> HMGAPATVTEQGEDITSKKDRGVLKIVKRVGNGEETPMIGDKVYVHYKGKLSNGKKFDSSHDRNEPFVFSLGKGQV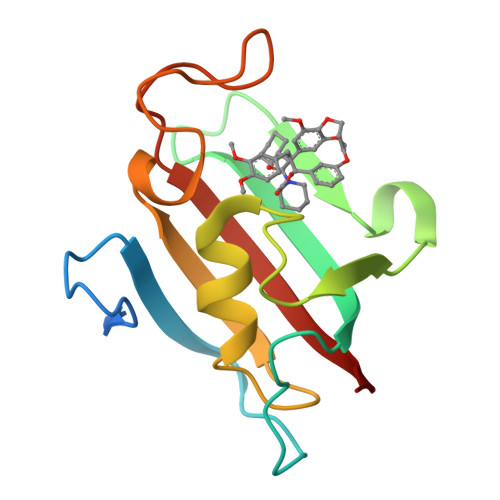IKAWDIGVATMKKGEIAHLLIKPEYAYGSAGSLPKIPSNATLFFEIELLDFKGE> MLQCYNC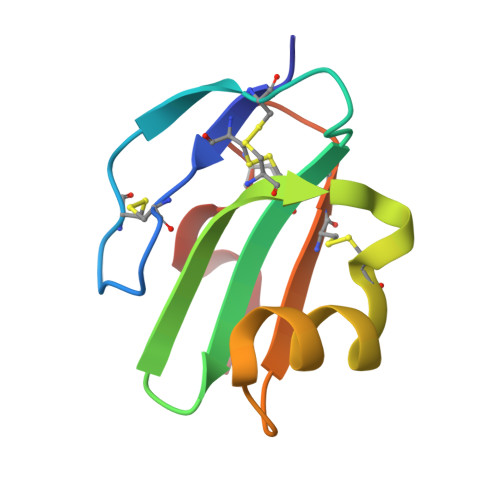PNPTADCKTAVNCSSDFDACLITKAGLQVYNKCWKFEHCNFNDVTTRLRENELTYYCCKKDLCNFNEQLEN Here we show that ubiquitin associated protein 1 (UBAP1), a subunit of human ESCRT-I, coassembles in a stable 1:1:1:1 complex with Vps23/TSG101, VPS28, and VPS37. The X-ray crystal structure of the C-terminal region of UBAP1 reveals a domain that we describe as a solenoid of overlapping UBAs (SOUBA). NMR analysis shows that each of the three rigidly arranged overlapping UBAs making up the SOUBA interact with ubiquitin. UBAP1's function is exclusively required for degradation of ubiquitinated endosomal cargo but not for other ESCRT-I-mediated processes such as midbody abscission or viral budding.

Two constructs covering the UBAP1 C terminus, residues 381–502 and 389–502, produced ample protein but did not crystallize. One of these mutants, with 415-KKGE-418 mutated to AAGA, readily crystallized. The 1.65 Å resolution crystal structure of the UBA-containing C-terminal region from UBAP1 has two molecules in the asymmetric unit that are linked to each other through a disulfide bond. However, multiangle laser light scattering indicates that the molecule is a monomer in solution (data not shown). It appears that the disulfide-linked dimer is formed as the protein oxidizes during the crystallization process. The structure shows a single domain consisting of seven α helices arranged as a right-handed solenoid that contains three overlapping UBAs (UBA1, UBA2, and UBA3). The relationship of the SOUBA fold to conventional UBAs can best be described by regarding the third helix of one UBAs being also the first helix of the next UBA. The solenoid arrangement of the three UBAs forms a convex surface containing helices one and three from each UBA. The opposite face forms a concave surface built from the second helix from each UBA. The residues showing the greatest perturbation lie along the convex face of the SOUBA domain and cover an extended hydrophobic surface.

>GSHMSPSERQCVETVVNMGYSYECVLRAMKAAGANIEQILDYLFAHGQLCEKGFDPLLVEEALEMHQCSEEKMMEFLQLMSKFKEMGFELKDIKEVLLLHNNDQDNALEDLMARAGAS[2x]(2R,3S,4R,5S)-2-(hydroxymethyl)piperidine-3,4,5-triol | C6 H13 N O4 | 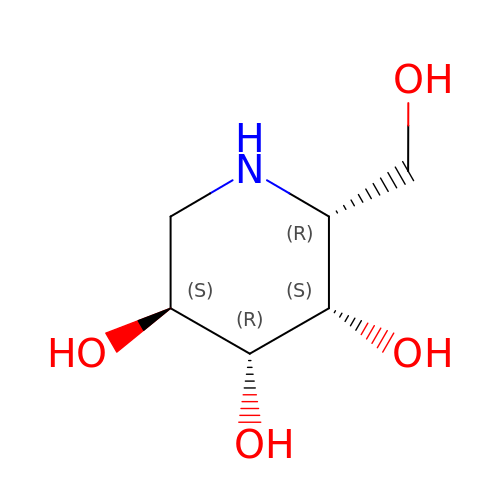LXBIFEVIBLOUGU-DPYQTVNSSA-N(5beta,9beta)-3-oxocholan-24-oic acid | C24 H38 O3 | 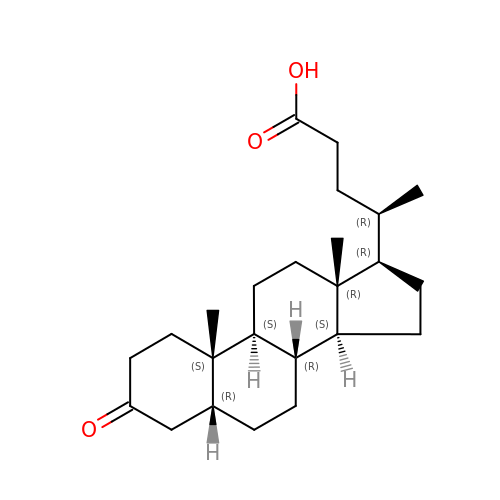KIQFUORWRVZTHT-OPTMKGCMSA-N> MENTENSVDSKSIKNLEPKIIHGSESMDSGISLDNSYKMDYPEMGLCIIINNKNFHKSTGMTSRSGTDVDAANLRETFRNLKYEVRNKNDLTREEIVEL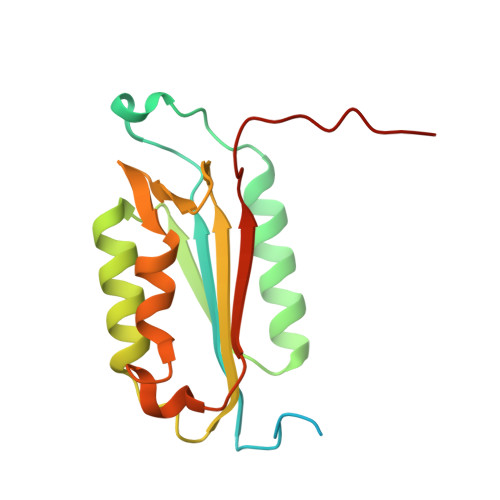MRDVSKEDHSKRSSFVCVLLSHGEEGIIFGTNGPVDLKKITNFFRGDRCRSLTGKPKLFIIQACRGTELDCGIETD>ACGLVASNLNLKPGECLKVRGELAPDAKSFVLNLGKDSNNLCLHFNPRFNAHGDANTIVCNSKDDGTWGTEQRETAFPFQPGSITEVCITFDQADLTIKLPDGHEFKFPNRLNMEAINYMAADGDFKIKCVAFE[8x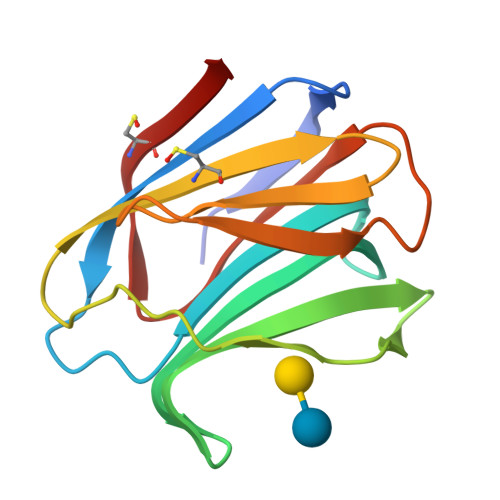]> MLDFFTIFSKGGLVLWCFQGVSDSCTGPVNALIRSVLLQERGGNNSFTHEALTLKYKLDNQFELVFVVGFQKILTLTYVDKLIDDVHRLFRDKYRTEIQQQSALSLLNGTFDFQNDFLRLLREAEESSKIRAPTTMKKFEDSEKAKKPVRSMIETRGEKPKEKAKNSKKKGAKKEGSDGPLATSKAVPAEKSGLPVGPENGVELSKEELIRRKREEFIQKHGRGLEKSSKSKSEAPKEKGKKAPRVWELGGCANKEVLDYSTPTTNGAPEAALSEDINLIRGTGPGGQLQDLDCSSSDDEGAAQNSTKPSSTKGTLGGMFGMLKGLVGSKSLSREDMESVLDKMRDHLIAKNVAADIAVQLCESVANKLEGKVMGTFSTVTSTVKQALQESLVQILQPQRRVDMLRDIMDAQRRQRPYVVTFCGVNGVGKSTNLAKISFWLLENGFSVLIAACDTFRAGAVEQLRTHTRRLSALHPPEKHGGRTMVQLFEK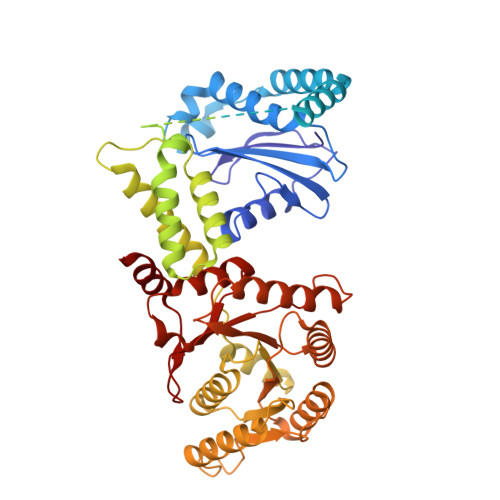GYGKDAAGIAMEAIAFARNQGFDVVLVDTAGRMQDNAPLMTALAKLITVNTPDLVLFVGEALVGNEAVDQLVKFNRALADHSMAQTPRLIDGIVLTKFDTIDDKVGAAISMTYITSKPIVFVGTGQTYCDLRSLNAKAVVAALMKA> MSKHCGLEANQKATDNEPKKRIRWNKSQRTLIEKLTADKHRKLRQSRRTADIYGDEVSAAQSQKLAEIEEVLIRSAGDVISLDRGQYDKWASLVSAKLGWRRGNPLNPSLNYSQAGEVREALKDARRVAQNLINDASHIRMLDGIKRFDDIYRQIMKPLGMTTDDARALFNETIEIGSIPKNNKIYGNSEGVRLINSLRHSDYIERAKGYGLNDEAIETLLRAATDVHSVFDEMRVIAEATGHNIEELQNLGYFPRIATRDFNIRLRKALETDTALADVIMSEGVEQVKALNPLSSVWQKSRKFNYFV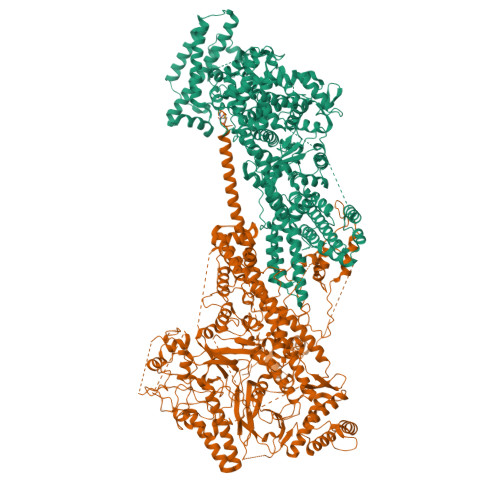PDDLEVASKLLNTSSDEIAEMLLNPREWMEFLTSSVSSSQIETMTELGVMSKLPMTSREVFEQLVDQYELPYKHINEMFKLDPHVAAEEYARVLRQAVGNSAMLKTVVKDGLAAGWAVPEKMLKDLSPKERANFVPLSFQKLDQFMSPEQLEAAGKVYVHRVVSDQWRSMLEISMSANKLGAFASAWSHLSTFLNKSVLASRNVLYVGTNFLSGFVLTNAVGANVFTVPHAMMDISNYLAKGLDAFDGTKPFAKIGGEWISKREFFKQFLLKRGSDITPGTVSTTSSGGDANPFTSFKSIGALADVRSAKRALEYLWSYSSSFGDPVRGTKGAAEYVGSLLNEATDNFFSPFAKMASFLDTMYKWNAYTSLVERQGAAELANTIAQGMTLEPISRIGRKFDNWRDLSRHIDDYFFTFDDPGTTTKVISKYVRPFANWSMQSTPAMLRAALRSPQKFSAYAKLLQLYNRGNNDDEPLNQSQLTDWQDDEYPVILQRDALQTGDGNGGLLVLFPHTFDPITDTLNVIDNAGRTVNILFGNKYGGNERDNRNSVTGKKDGLTSMLTELFNDTYWAKPAGLLLGIDSFTGQKIDASKYNNYLGFEMHPLAEALLGMYTPLDAINRTNLFDTFGRREYKDYRDRTVVEEKPGLFGGQRTNSDAQSLAWETAVKNGNWSALALMTMGARVRLIDTARNTQMTLDEIKTGIDELQKANVNAARQLTLNPEKLSESERNKRTERLTESLTAEYQMKYDYARLINYMKAKRIPPKRLLFEMQQRSVNVSDLEPVGGKQRLQLESDFRRRIEEINK;> MSIIKDVQDSNDPQLDKFNNEDAPKLAPVIPTPQPTDAGLSLGSTPVGVNPQAVIETESTPQPLTPEQQALTDSYNEASRLTTNVQPMSELVQPQQALPTPTNIDSQQPTVFESANQFNLSATDNLLQQGKITQELINETQLTQSHIPTVYSTPYDGDEWDLDFEASLERAGVLPGQKPSPETFNSQFNAQPTNEDASRSFNPNALKRSQFDVEGALAAIRNINTQEGLTGYQTIKPWGEGALSSLMYGLGVVSNTIRGGVIDAVNVRNRVVNQLPKPIQGVLNFNPASALTGQQLIRPDANYRGSYTLDAIRGRQYSFTANSTNKDEPIGITGFKAFDDLAERMRQNRNARYNAINKTFGREIAKPVAVEERWSTDLSFWAGFGLDTILDPIDSIGVAWKASGLLLGNAPSYVKRGIPTNTGRVIVTPAASERKLLPPGRTRYTPPGKPDGYELGLTEPLTNNKYQVVQTPKGEVSIPVGQPTVQAKLPSIASNNKVTSLTLRREIRRPDGVIDVEFTPNPGAFDRVTGISNEPLAQLPSSEARRPLEPTQFETIQTPNGEVQVPINQPSAPRQLPGTRTYSQPNWRWSRVVDGYINPEGMQPIIEVVRRKPEVFTTNSTSGYSPNWEYWSAPKVDDLYIPAPIDVEFKVIPNKPSNLPLKPSSLSEDIVQGVDGEVRVPSSTQPNSQLALPYGEPYPLTQWDLSLETNPPQIGQRIDNNITVAKNQGEAIDDVINNAPRTVEYNVSGLEIPRRNVTPQGFPKLEPRYDIKPPETPRVIELAPESVTVIREALDSNDWVKAYDELLRKRVPVSDIKRKLETGRIDEAVNDLRKLIGDIKPKTAPEPKPVAPKRQRRRVIKADGTAVYETVRVNPETQLLDAAITNINVVANVVDVPSMSVSQSTPASPLAIDAASDALRPVSPGTPLVAPTSEVNKQLVDQLTRLTETERMMKRRGASPETLERIRTQKLELRKAIADGDELAEPKVKPEPVTPAINKTVLTGTMTMSELSQQLLDNVPGSRIDPDKVRRVERKLSEVEALMKVIPNPITGEPLLGSANTRKFRTWAKDSSTSPTAYLNKLGLQEYPLLYRLFERDGAAIDIDALAHPEFRVILDKPLPDKTSRQVVVSNTPSLTKPTVQSESKAITEMTINELRSERKLLKSQINELDDPSDLIERLMELDDAINNLDITKPENLKVVQDEVIPETQHGTSPEVVKLTQQKLDIENEVINTGVRVQELELELARQKVQLEDALSRIEETADINPHDVISEPLPSGRARRVPTEIPPNDGTILTQKEAARFYDISEGNFKNGDTKPRPALVHTKHMVSDVVVPNDVIQREFDNIMNMGGITQPIVITPVGLDDVYIKYAVVDNHAIYEAAKLAREADPRKFENVNVIVIHPSKADPSYFADEVLPTNTTEGSLYHGTRVKGWTPGNGGVGEWGSGTYFSKSSQAASDNAIKPLRPALGEVIDNVTQPTIHEVLPDFKRTVDVNSPVDGDFSAALLMSANELMDGSEFTSFKRSIMKPGTVQLRDTIKTPADIYAAIEKYAAKNDIEWTPERTHKFKSRINERLRLVGVDALTDGDTTLVINPDAVSVINSHLLDETDAIGTSIARYNSASEAAGRNSGIPTANANQAEASVMLQRQMYEETIEKLEDAKRQQRTAITKSHEIDEQLTQTAQAEQTTKRQQRVAKSQKRAEREAERLGKKRDNPCQF>[2x]MKEFYLTVEQIGDSIFERYIDSNGRERTREVEYKPSLFAHCPESQATKYFDIYGKPCTRKLFANMRDASQWIKRMEDIGLEALGMDDFKLAYLSDTYNYEIKYDHTKIRVANFDIEVTSPDGFPEPSQAKHPIDAITHYDSIDDRFYVFDLLNSPYGNVEEWSIEIAAKLQEQGGDEVPSEIIDKIIYMPFDNEKELLMEYLNFWQQKTPVILTGWNVESFAIPYVYNRIKNIFGESTAKRLSPHRKTRVKVIENMYGSREIITLFGISVLDYIDLYKKFSFTNQPSYSLDYISEFELNVGKLKYDGPISKLRESNHQRYISYNIIAVYRVLQIDAKRQFIN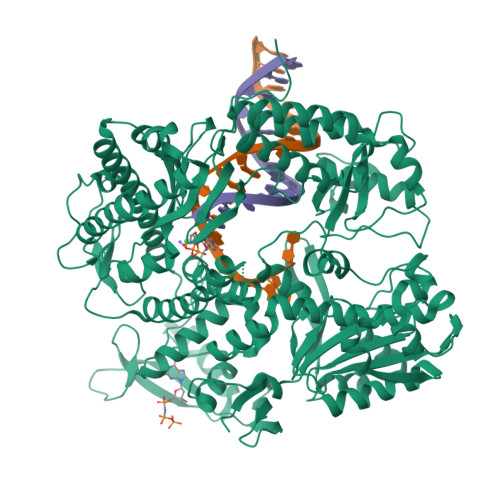LSLDMGYYAKIQIQSVFSPIKTWDAIIFNSLKEQNKVIPQGRSHPVQPYPGAFVKEPIPNRYKYVMSFDLTSLYPSIIRQVNISPETIAGTFKVAPLHDYINAVAERPSDVYSCSPNGMMYYKDRDGVVPTEITKVFNQRKEHKGYMLAAQRNGEIIKEALHNPNLSVDEPLDVDYRFDFSDEIKEKIKKLSAKSLNEMLFRAQRTEVAGMTAQINRKLLINSLAGALGNVWFRYYDLRNATAITTFGQMALQWIERKVNEYLNEVCGTEGEAFVLYGDTDSIYVSADKIIDKVGESKFRDTNHWVDFLDKFARERMEPAIDRGFREMCEYMNNKQHLMFMDREAIAGPPLGSKGIGGFWTGKKRYALNVWAMEGTRYAEPKLKIMGLETQKSSTPKAVQKALKECIRRMLQEGEESLQEYFKEFEKEFRQLNYISIASVSSANNIAKYDVGGFPGPKCPFHIRGILTYNRAIKGNIDAPQVVEGEKVYVLPLREGNPFGDKCIAWPSGTEITDLIKDDVLHWMDYTVLLEKTFIKPLEGFTSAAKLDYEKKASLFDMFDF> MTVFRQENVDDYYDTGEELGSGQFAVVKKCREKSTGLQYAAKFIKKRRTKSSRRGVSREDIEREVSILKEIQHPNVITLHEVYENKTDVILIGELVAGGELFD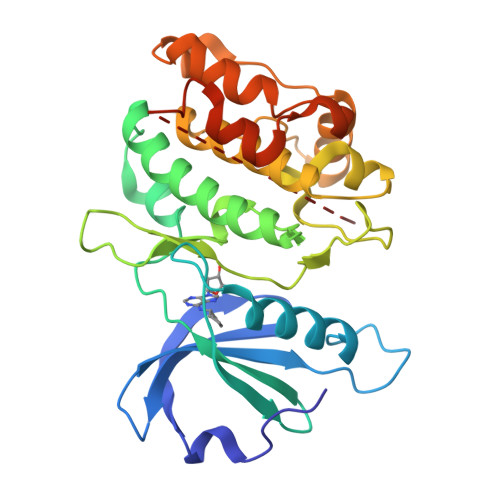FLAEKESLTEEEATEFLKQILNGVYYLHSLQIAHFDLKPENIMLLDRNVPKPRIKIIDFGLAHKIDFGNEFKNIFGTPEFVAPEIVNYEPLGLEADMWSIGVITYILLSGASPFLGDTKQETLANVSAVNYEFEDEYFSNTSALAKDFIRRLLVKDPKKRMTIQDSLQHPWIKPKDTQQALSSAWSHPQFEK> VNINILQQIGYIKQQVRQLSYYSQSSSSYIVVKLLPNIQPTDDSCEFKSVTQYNKTLSNLLLPIAENINNIAIGIAALGVATAAQVTAAVSLVQAQTNARAIAAMKNSIQATNRAVFEVKEGTQQLAIAVQAIQDHINTIMNTQLNNMSCQILDNQLATSLGLYLTELTTCFQPQLTNPALSPISIQCLRSLLGSMTPAVVQATLSTSISAAEILSAGLMEGQIISVLLDEMQMIVKINIPTIVTQSNALVIDFYSISSFINNQESIIQLPDRILEIGNEQWSYPAKNCKLTRHHIFCQYNEAERLSLESKLCLAGNISACVFSPIAGSYMRRFVALDGTIVANCRSLTCLCKSPSYPIYQPDHHAVTTIDLTACQTLSLDGLDFSIVSLSNITYAENLTISLSQTINTQPIDISTELSKVNASLQNAVKYIKESNHQLQS

Neutralization titers elicited by paramyxovirus Pre-F glycoproteins are more potent than those elicited by their Post-F counterparts; therefore, we aimed to develop a prefusion-stabilized mumps F glycoprotein trimer. Structural engineering of F and HN glycoproteins has led to the identification of prefusion-stabilized F and chimeric immunogens that elicit high-titer neutralizing antibodies to diverse mumps viruses in mice compared to titers routinely observed following MMR vaccination in humans. These Pre-F and Pre-F/HN chimeric glycoproteins are promising primary series or booster vaccine candidates for mumps.

Here, we report the design, crystal structure to 2.16 Å resolution of a mumps genotype G Pre-F glycoprotein trimer, and the engineering of a chimeric mumps Pre-F trimer fused with mumps genotype G HN head domain (Pre-F/HN). By creating a matrix of disulfide substitutions and C-terminal coiled-coil-GCN4 attachment positions while mutating cleavage site residues 101–103 to three glycine residues (Gly3), we evaluated the level of protein expression and the proportion of protein adopting the prefusion or postfusion conformation using NS-EM. While five combinations of disulfide bonds, cleavage site mutations, and GCN4 attachment positions gave rise to 100% prefusion trimers, only one such combination resulted in high-yield protein expression (V206C-A223C with 476-GCN4 and 101KRF-101GGG) at about 4.8 mg/L from Expi293 cells. Size-exclusion chromatography of mumps Pre-F revealed a single peak which, when expressed in the presence of kifunensine and the 6 potential N-linked glycosylation sites (PNGS) per protomer enzymatically deglycosylated (Pre-F-Δglycan), could be crystallized. The x-ray structure to 2.16 Å resolution revealed a similar overall architecture to PIV5 and other paramyxovirus Pre-F trimers. However, the apex of the mumps prefusion F trimer adopts a “closed cap” structure comprising loops N177-S184 formed by interactions between side chains T178, Q179, and N181, which has not been observed in other paramyxovirus Pre-F structures. The remaining N-acetyl glucosamine moieties from the six glycans at positions N73, N182, N352, N427, N433, and N457 were visible in the electron density maps and a Man5 glycosylated model built. The DI–DIII domains enclosed a large aqueous cavity measuring ~17,000 Å3 in volume and protomers bury a 6,500 Å2 interface, similar to that observed in PIV5, PIV3, Nipah, measles, and Langya Pre-F structures. Mapping the variation to Pre-F for all genotypes and specifically between genotype G and Jeryl Lynn (genotype A), much of the protein surface exposed for antibody recognition was conserved, while numerous variable amino acids were located within the aqueous cavity in the core of the prefusion trimer.> EFPHNAIEPCVICQTRPKNGCIVHGKTGHLMACFTCAKKLKKRNKPCPVCRQPIQMIVLTYFP;>[2x]EIVEPEFPHNAIEPCVICQTR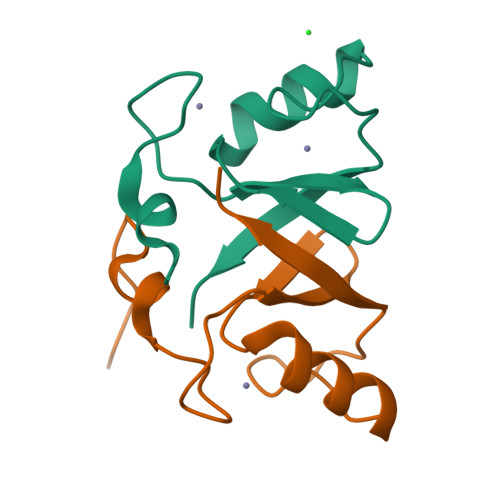PKNGCIVHGKTGHLMACFTCAKKLKKRNKPCPVCRQPIQMIVLTYFP;> EPEFPHNAIEPCVICQTRPKNGCIVHGKTGHLMACFTCAKKLKKRNKPCPVCRQPIQMIVLTYFP>DSFIRQHLRKLAPYQPILPFEVLSSRLGRKPEDIVKLDANENPYGPPPEVMEALGSIRFP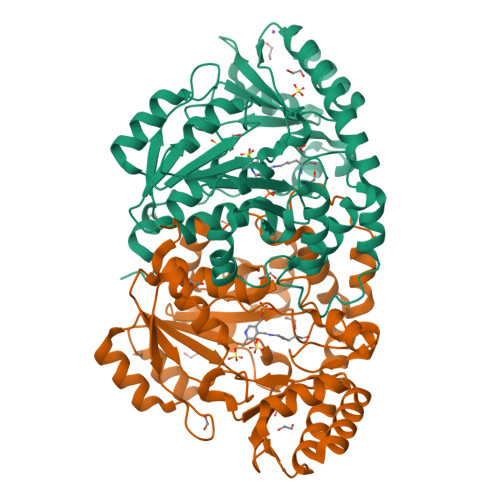YVYPDPESRRLRAALAQDSGLESEYILVGCGADELIDLIMRCVLDPGDKIVDCPPTFTMYEFDAAVNGALVIKVPRRPDFSLNVEQIIEVVKQEKPKCIFLTSPNNPDGSIIDDDDLLKILELPILVVLDEAYIEFSTIESKMSWVKKHDNLIVLRTFSKRAGLAGLRVGYGAFPLSIIKYLWRAKQPYNVSVAAEISACAALQNPTYLENVKDALVKERGRLFDLLKAVPFLKPFPSHSNFILCEVTSGVDPKKLKEDLAEMGVMIRHYSNKELKGYVRVSVGKPEHTDVLMNCISRLS[2x]> MKKKWYIVLTMSGYEEKVKENIEKKVEATGIKNLVGRIVIPEEVVLDATSPSERLILSPKAKLHVNNGKDVNKGDLIAEEPPIYARRSGVIVDVKNVRKIVVETIDRKYTKTYYIPESAGIEPGLRVGTKVKQGLPLSKNEEYICELDGKIVEIERMKKVVVQTPDG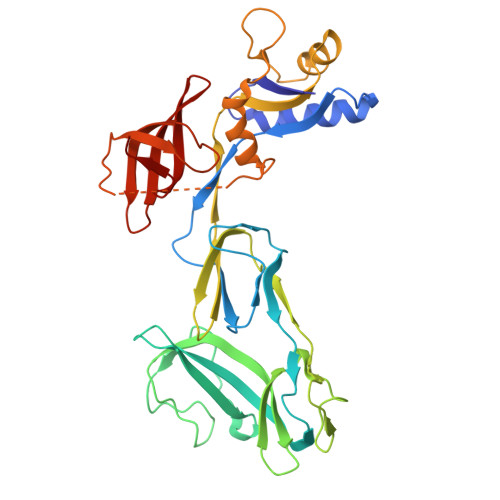EQDVYYIPLDVFDRDRIKKGKEVKQGEMLAEARKFFAKVSGRVEVVDYSTRKEIRIYKTKRRKLFPGYVFVEMIMNDEAYNFVRSVPYVMGFVSSGGQPVPVKDREMRPILRLAGLEEYEEKKKPVKVELGFKVGDMVKIISGPFEDFAGVIKEIDPERQELKVNVTIFGRETPVVLHVSEVEKI16,17-ANDROSTENE-3-OL | 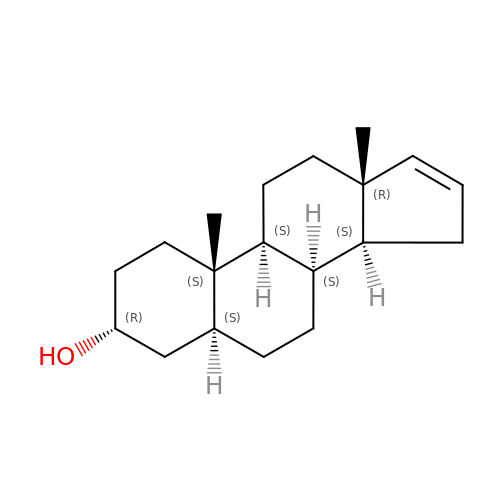C19 H30 O | KRVXMNNRSSQZJP-PHFHYRSDSA-N> MGSSHHHHHHSSGLVPRGSHMSSDSSVAASAQPPIAAKKPHRVTLGYVEGEDRGPNPMNPPRYREDPYFWMRDDDRKDPAVIEHLNKEKVYFQARSADIAQLRDDIYAEHISHINEDDMSAPYVYGKYRYYTREVKGKPYKIYCRVFTDKEPGDVAAEEVIIDVNQVAEGKAFCD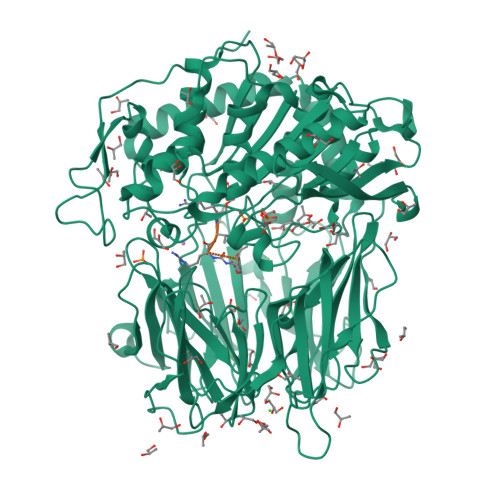VMEVKPAPPEHDLVAFSVDMSGNEVYTIEFKRISDPSQTIADKVSGTNGEIVWGPDHTSLFYVTKDETLRENKVWRHVMGKLQSEDVCLYEEHNPLFSAFMYKAADTNTLCIGSQSPETAEVHLLDLRKGNAHNTLEIVRPREKGVRYDVQMHGTSHLVILTNEGGAVNHKLLIAPRGQPSDWSHVLVDHSEDVFMESIAVRSNYLVVAGRRAGLTRIWTMMADSQDGVFKAGTGLREVVMEEPIFTVHLVESQMLEYEEPTFRMEYSSLATPNTWFDVSPQDHSRTAVKVREVGGGFDAANYKVERRFATAPDQTKIPLSVVYHKDLDMSQPQPCMLYGYGSYGLSMDPQFSIQHLPYCDRGMIFAIAHIRGGSELGRAWYEIGAKYLTKRNTFSDFIAAAEFLVNAKLTTPSQLACEGRSAGGLLMGAVLNMRPDLFKVALAGVPFVDVMTTMCDPSIPLTTGEWEEWGNPNEYKYYDYMLSYSPMDNVRAQEYPNIMVQCGLHDPRVAYWEPAKWVSKLRECKTDNNEILLNIDMESGHFSAKDRYKFWKESAIQQAFVCKHLKSTVRLLVRR;> FRVR(2~{S},3~{R},4~{S},5~{S},6~{R})-2-ethoxy-6-(hydroxymethyl)oxane-3,4,5-triol | C8 H16 O6 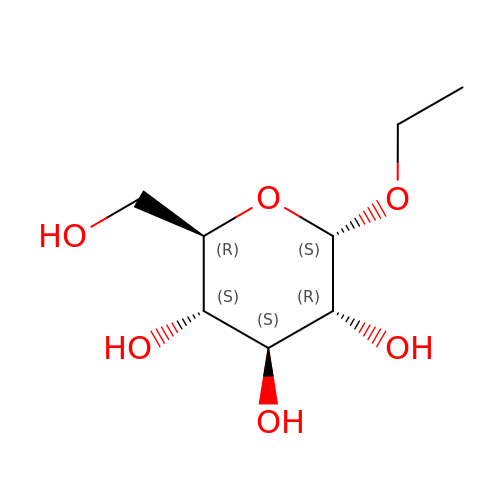| WYUFTYLVLQZQNH-CBQIKETKSA-N>[3x]MKYDTSELCDIYQEDVNVVEPLF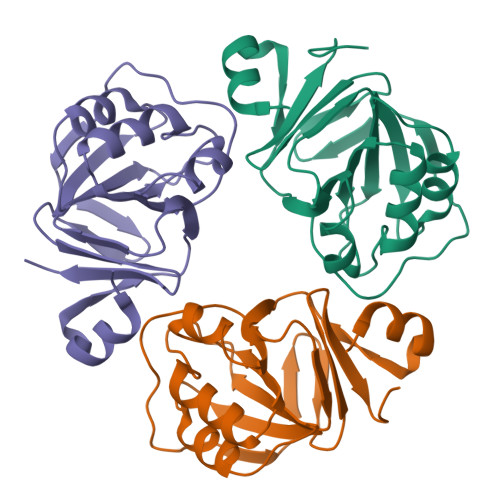SNFGGRASFGGQIITVKCFEDNGLLYDLLEQNGRGRVLVVDGGGSVRRALVDAELARLAVQNEWEGLVIYGAVRQVDDLEELDIGIQAMAAIPVGAAGEGIGESDVRVNFGGVTFFSGDHLYADNTGIILSEDPLDIE> GSTPIPAMQAALAATDLDGWLVYDFQGLNPHARRVLGIGDDVFLTRRFFVWVPRAGRAVVLHNHIEGGNWNRITQEWDAELRPFGSHAELDAALRGVVSGQRLAMEYSPNGAVPYVSRVDAGTLERVRGAGAAEVASSADLLQAFLVWTPDDLAAHRRAAALLMRAKDDAFRLIHDRLRAGQSVTEWEVQQLIMDQIRAAGMQAGHDVNVSFGVNAADSHYEPSEQRSATLHPGECVLIDLWAQEPGRPFADVTWVGFAGEPGTEYLDAWQAVRAAREAALELLRSRFVAEGYGRLQGWELDRAARDAMGERWAPHFLHRTGHDLGVQIHGAGANLD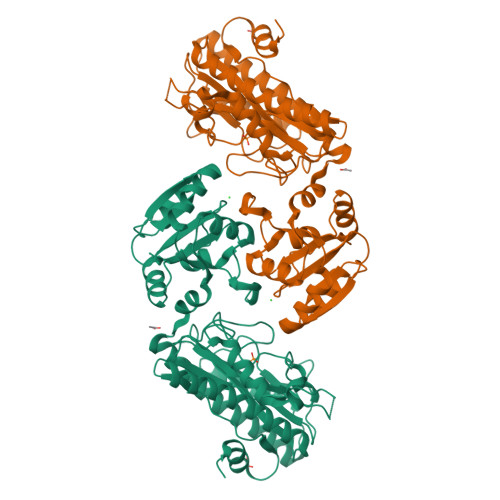DYETRDTRTLTPGLSVTVEPGTYPAAASPSGQGGFGIRSEVDVYLAPDGPEVTTDLQQAPFILGVGDWDAVRAAGYGEQ>MATLTAKNLAKAYKGRRVVEDVSLTVNSGEIVGLLGPNGAGKTTTFYMVVGIVPRDAGNIIIDDDDISLLPLHARARRGIGYLPQEASIFRRLSVYDNLMAVLQIRDDLSAEQREDRANELMEEFHIEHLRDSMGQSLSGGERRRVEIARALAANPKFILLDEPFAGVDPISVIDIKRIIEHLRDSGLGVLITDHNVRETLAVCERAYIVSQGHLIAHGTPTEILQDEHVKRVYLGEDFRL[2x];> MIIIRYLVRETLKSQLAILFILLLIFFCQKLVRILGAAVDGDIPANLVLSLLGLGVPEMAQLILPLSLFLGLLMTLGKLYTESEITVMHACGLSKAVLVKAAMILAVFTAIVAAVNVMWAGPWSSRHQDEVLAEAKANPGMAALAQGQFQQATNGSSVLFIESVDGSDFKDVFLAQIRPKGNARPSVVVADSGHLTQLRDGSQVVTLNQGTRFEGTALLRDFRITDFQDYQAIIGHQAVALDPNDTDQMDMRTLWNTDTDRARAELNWRITLVVTVFMMALMVVPLSVVNPRQGRVLSMLPAMLLYLLFFLIQTSLKSNGGKGKLDPTL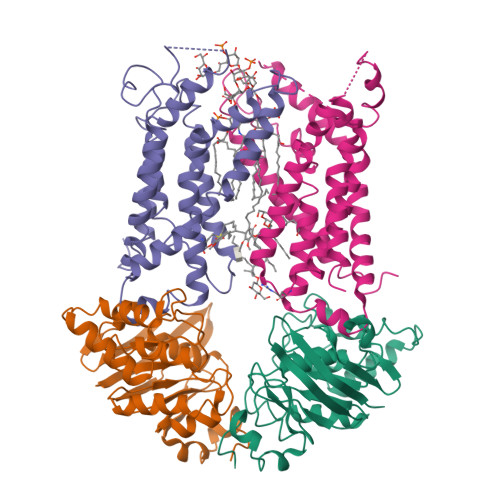WMWTVNLIYLALAIVLNLWDTVPVRRLRASFSRKGAV;> MQPFGVLDRYIGKTIFTTIMMTLFMLVSLSGIIKFVDQLKKAGQGSYDALGAGMYTLLSVPKDVQIFFPMAALLGALLGLGMLAQRSELVVMQASGFTRMQVALSVMKTAIPLVLLTMAIGEWVAPQGEQMARNYRAQAMYGGSLLSTQQGLWAKDGNNFVYIERVKGDEVLGGISIYAFNENRRLQSVRYAATAKFDPEHKVWRLSQVDESDLTNPKQITGSQTVSGTWKTDLTPDKLGVVALDPDALSISGLHNYVKYLKSSGQDAGRYQLNMWSKIFQPLSVAVMMLMALSFIFGPLRSVPMGVRVVTGISFGFVFYVLDQIFGPLTLVYGIPPIIGALLPSASFFLISLWLLMRKS>[5x]DTTQPALLRLSDHLLANYKKGVRPVRDWRKPTTVSIDVIMYAILNVDEKNQVLTTYIWYRQYWTDEFLQWTPEDFDNVTKLSIPTDSIWVPDILINEFVDVGKSPNIPYVYVHHRGEVQNYKPLQLVTACSLDIYNFPFDVQNCSLTFTSWLHTIQDINITLWRSPEEVRSDKSIFINQGEWELLEVFPQFKEFSIDISNSYAEMKFYVIIRRRPLFYAVSLLLPSIFLMVVDIVGFCLPPDSGERVSFKITLLLGYSVFLIIVSDTLPATAIGTPLIGVYFVVCMALLVISLAETIFIVRLVHKQDLQRPVPDWLRHLVLDRIAWILCLGEQPMAHRPPATFQANKTDDCSGSDLLPAMGNHCSHVGGPQDLEKTPRGRGSPLPPPREASLAVRGLLQELSSIRHFLEKRDEMREVARDWLRVGYVLDRLLFRIYLLAVLAYSITLVTLWSIWHYS

The ion channel class of serotonin receptors (5-HT3AR) are cation selective and belong to the super family of pentameric ligand-gated ion channels (pLGICs). The 5-HT3AR pentameric complex is ~250 KDa in molecular weight and is made up of five homologous subunits A (5-HT3A) or a heterologous combination of subunit A with other subunits (B–E) arranged around a pseudo five-fold symmetric axis. At the structural level, 5-HT3AR is a dynamic allosteric protein where binding of the neurotransmitter serotonin in the N-terminal extracellular domain (ECD) elicits a conformational change leading to pore opening within the transmembrane domain (TMD). In addition to these two domains, the channel has a large intracellular domain (ICD) formed by the region between the transmembrane M3 and M4 helices.

The cryo-EM structure of apo-5-HT3AR at 4.3 Å resolution is similar to the 5-HT3AR crystal structure but is captured in a distinct state with differences in the ECD, TMD, and the ICD conformations. An alignment of the two structures reveals an expansion of all the three domains in apo-5-HT3AR resulting from a radial outward twist of the ECD outer β-sheet and an iris-like movement of the TM helices and the ICD. In addition, Loop C, which is at the periphery of the neurotransmitter binding pocket, in the apo-5-HT3AR structure is placed outward in an open or “extended” conformation. Further down, the pore at Leu9′ is constricted to ~2.3 Å which is too small to allow a hydrated Na+35 to pass through and in addition the hydrophobicity of this region prevents ion dehydration. The intracellular end is lined by two rings of negative charges at positions Glu-1′ and Asp-4′ which are involved in governing charge selectivity and constitute the selectivity filter. This suggests that the channel in this conformation is non-conducting and the Leu9′ position acts as a gate impeding ion permeation. The ICD reveals a notable constriction to 2.1 Å at the level of Arg416 with a strong density (6 σ) at the center of the pore axis, which we modeled as a Cl−. At the edge of the TMD–ICD interface, there is a density present in the cavity lined by M3 of one subunit and M1 and M4 helices of the neighboring subunit. This density was partially modeled as a phospholipid based on putative polar contacts with neighboring Arg sidechains (Arg306 in M3 and Arg435 in M4). The mouse 5-HT3AR has three N-glycosylation sites at positions Asn82, Asn148, and Asn164, and strong densities for glycans were observed at each of the asparagine sidechains. Based on these distances, the pore radii at this location (>hydrated Na+ ion radius), and the B-factors for the modeled ions and waters, we suggest that these densities likely correspond to ions and water. The cryo-EM structure of apo-5-HT3AR determined in the solution state, in the absence of inhibitors, Fab fragments, truncation, or constraints from crystal lattice, bears the hallmarks of the resting conformation.5-(1-tert-butyl-1H-pyrazol-4-yl)-7-oxo-6-(propan-2-yl)-4,7-dihydropyrazolo[1,5-a]pyrimidine-3-carbonitrile 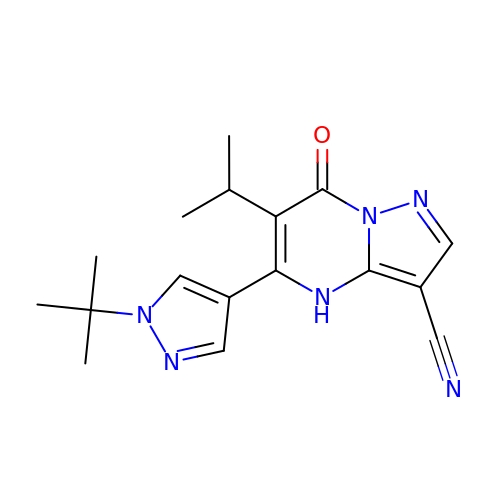| C17 H20 N6 O | KRXWJZIHQRIGSJ-UHFFFAOYSA-N> TTLLNPYFGEFGGMYVPQILMPALNQLEEAFVSAQKDPEFQAQFADLLKNYAGRPTALTKCQNITAGTRTTLYLKREDLLHG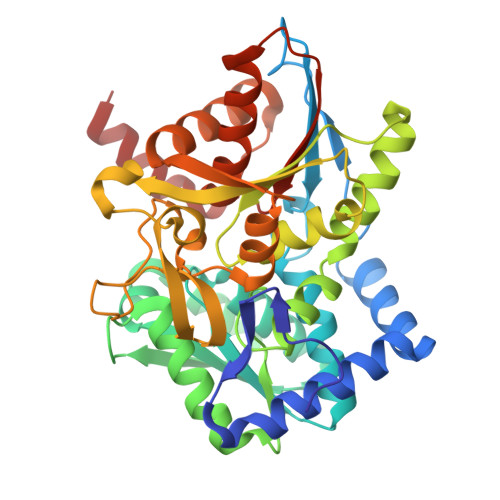GAHKTNQVLGQALLAKRMGKSEIIAETGAGAHGVASALASALLGLKCRIYMGAKDVERQSPNVFRMRLMGAEVIPVHSGSATLKDACNEALRDWSGSYETAHYMLGTAAGPHPYPTIVREFQRMIGEETKAQILDKEGRLPDAVIACVGGGSNAIGMFADFINDTSVGLIGVEPGGHGIETGEHGAPLKHGRVGIYFGMKAPMMQTADGQIEESYSISAGLDFPSVGPQHAYLNSIGRADYVSITDDEALEAFKTLCRHEGIIPALESSHALAHALKMMREQPEKEQLLVVNLSGRGDKDIFTVHDILKARG>MGSSHHHHHHSSGRENLYFQGAKKSIYDYTDEEKVQSAFDIKEEGNEFFKKNEINEAIVKYKEALDFFIHTEEWDDQILLDKKKNIEISCNLNLATCYNKNKDYPKAIDHASKVLKIDKNNVKALYKLGVANMYFGFLEEAKENLYKAASLNPNNLDIRNSYELCVNKLKEARKKDKLTFGGM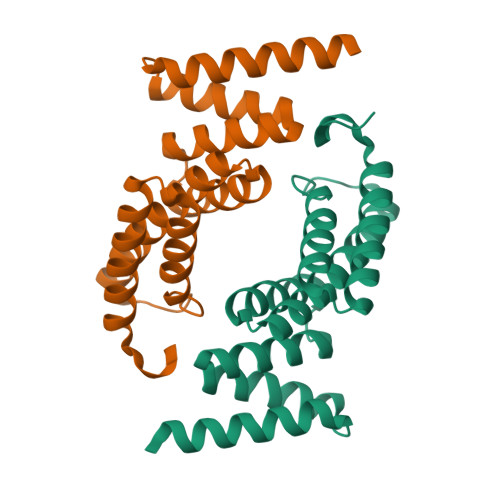FDKGPLYEEKKNSAN[2x]ME-A-9-N-(BIPHENYL-4-CARBONYL)-AMINO-9-DEOXY-NEU5AC | C25 H30 N2 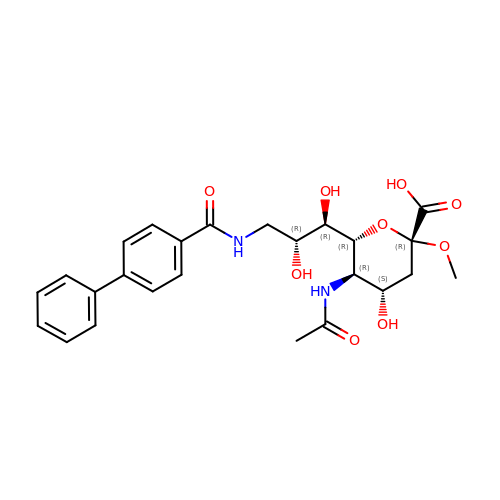O9 | WBWCOQWBSRYCDR-TUTCKEIYSA-N> GPGYQEELLQASVSPYHLFSDVADVTAFRSNLLSWYDQEKRDLPWRNLAKEEANSDRRAYAVWVSEVMLQQTQVATVIDYYTRWMQKWPKLQDLASASLEEVNQLWSGLGYYSRGRRLQEGARKVVEELGGHMPRTAETLQQLLPGVGRYTAGAIASIAFDQVTGVVDGNVLRVLCRVRAIGADPTSTLVSHHLWNLAQQLVDPARPGDFNQAAM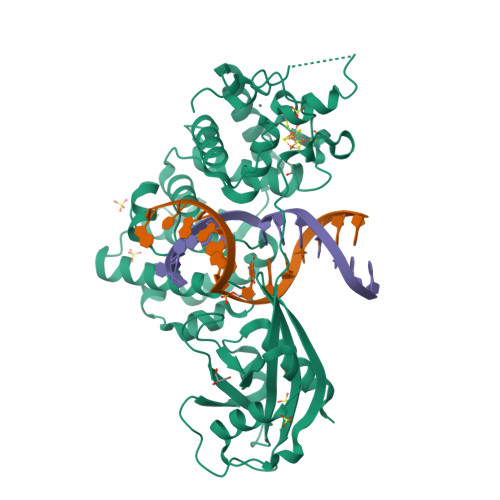ELGATVCTPQRPLCSHCPVQSLCRAYQRVQRGQLSALPGRPDIEECALNTRQCQLCLTSSSPWDPSMGVANFPRKASRRPPREEYSATCVVEQPGAIGGPLVLLVQRPDSGLLAGLWEFPSVTLEPSEQHQHKALLQELQRWCGPLPAIRLQHLGEVIHIFSHIKLTYQVYSLALDQAPASTAPPGARWLTWEEFCNAAVSTAMKKVFRMYEDHRQGTRKGSKRSQVCPPSSR> LRRSNRWCMKYANLE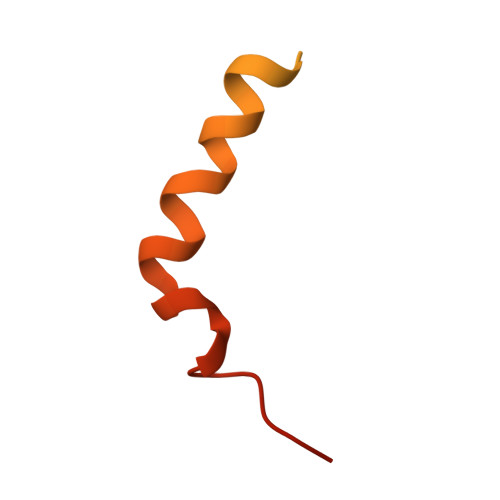LTTRGEFPHGMKEPGFVKKLDKNIPWYFSTYRSMYHWPVAGDGWSDLNEAEKHHDLHMYYTLAWWKLGEGIFDADDEDR> RSKSDG;> GSHMPPNRPGITFEIGARLEALDYLQKWYPSRIEKIDYEE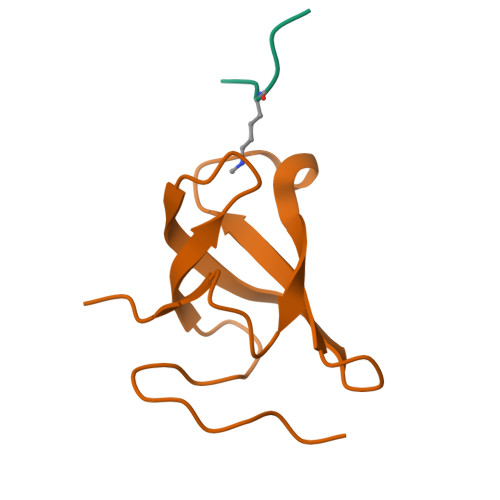GKMLVHFERWSHRYDEWIYWDSNRLRPLER>[2x]MELWLVRHGETLWNREGRLLGWTDLPLTAEGEAQARRLKGALPSLPAFSSDLLRARRTAELAGFSPRLYPEMREIHFGALEGALWETLDPRYKE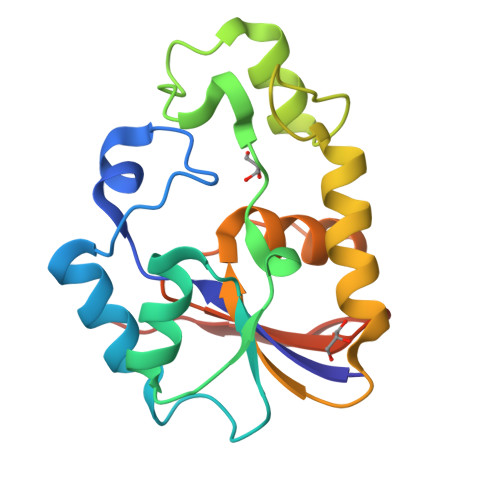ALLRFQGFHPPGGESLSAFQERVFRFLEGLKAPAVLFTHGGVVRAVLRALGEDGLVPPGSAVAVDWPRRVLVRLALDGEEATG>SMVEVLADHPGELVRTDSPNFLCSVLPTHWRCNKTLPIAFKVVALGDVPDGTLVTVMAGNDENYSAELRNATAAMKNQVARFNDLRFVGRSGRGKSFTLTITVFTNPPQVATYHRAIKITVDGPREPRRHRQKL[6x];>PRVVPDQRSK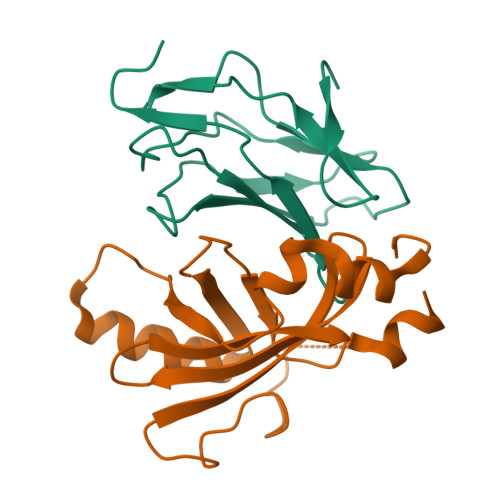FENEEFFRKLSRECEIKYTGFRDRPHEERQARFQNACRDGRSEIAFVATGTNLSLQFFPASWQGEQRQTPSREYVDLEREAGKVYLKAPMILNGVCVIWKGWIDLQRLDGMGCLEFDEERAQQE[4x]5-HYDROXY-L-TRYPTOPHAN 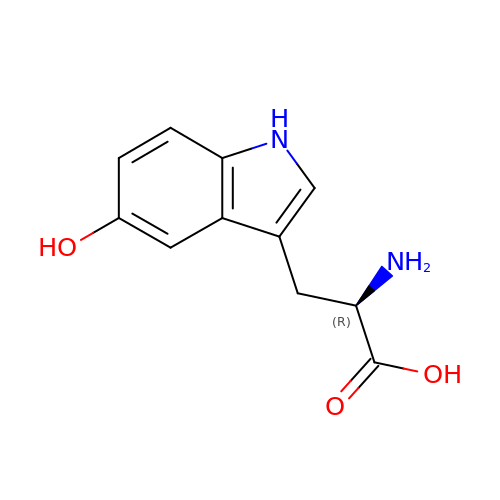| C11 H12 N2 O3 | LDCYZAJDBXYCGN-SECBINFHSA-N> GA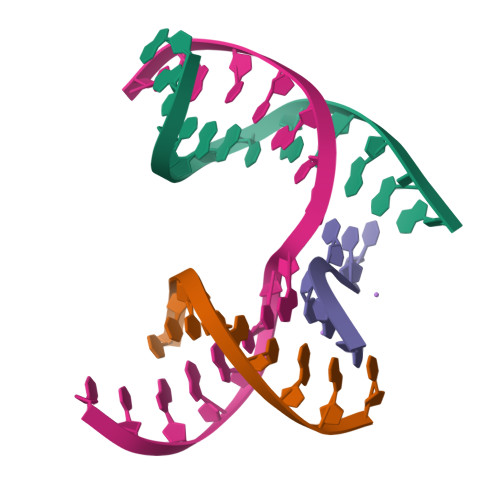ACGACACAGA;> CGACGACTC;> TCTTCG;> TCGAGTCGGTGTCGT>MGKKVAIIGAGVSGLASIRSCLEEGLEPTCFERSDDIGGLWKFSDHAEEGRASIYQSVFTNSSKEMMCFPDFPYPDDFPNFMHNSKLQEYITAFAKEKNLLKYIQFKTLVSSVNKRPDFSVTGQWD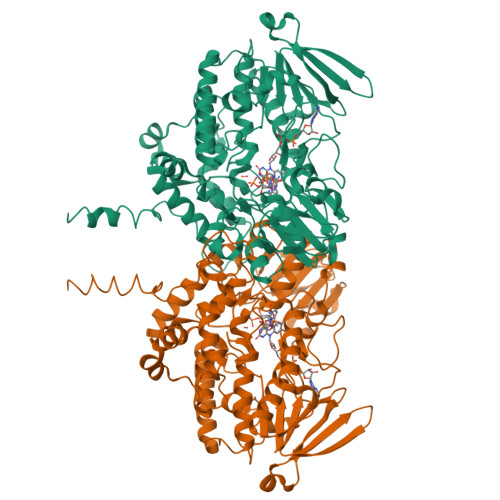VTTEKDGKKESAVFDAVMICSGHHVYPNLPKESFPGLKHFKGKCFHSRDYKEPGIFKGKRVLVIGLGNSGCDIATELSHTAEKVIISSRSGSWVMSRVWDDGYPWDMLFITRFETFLKNSLPTAISDWWYMKQMNARFKHENYGLMPLNGTLRKEPVFNDELPARILCGTVSIKPNVKEFTETSAIFEDGTVFEAIDCVIFATGYGYAYPFLDDSIIKSRNNEVTLFKGIFPPLLEKPTLAVIGLVQSLGATIPTTDLQARWAAKVFANSCTLPTTNEMMDDIDEKMGKKLKWFGQSQTLQTDYITYMDELGSFIGAKPNIPWLFLTDPQLALEVFFGPCSPYQFRLMGPGKWDGARNAILTQWDRTLKPTRTRAVGEAKRPSLFYNLLKILLFPVLLLAVLLAFY[6x]> ARPCIPKSFGYSSVVCVCNATYCDSFDPPTFPALGTFSRYESTRSGRRMELSMGPIQANHTGTGLLLTLQPEQKFQKVKGFGGAMTDAAALNILALSPPAQNLLLKSYFSEEGIGYNIIRVPMASCDFSIRTYTYADTPDDFQLHNFSLPEEDTKLKIPLIHRALQLAQRPVSLLASPWTSPTWLKTNGAVNGKGSLKGQPGDIYHQTWARYFVKFLDAYAEHKLQFWAVTAENEPSAGLLSGYPFQCLGFTPEHQRDFIARDLGPTLANSTHHNVRLLMLDDQRLLLPHWAKVVLTDPEAAKYVHGIAVHWYLDFLAPAKATLGETHRLFPNTMLFASEACVGSKFWEQSVRLGSWDRGMQYSHSIITNLLYHVVGWTDWNLALNPEGGPNWVRNFVDSPIIVDITKDTFYKQPMFYHLGHFSKFIPEGSQRVGLVASQKNDLDAVALMHPDGSAVVVVLNRSSKDVPLTIKDPAVGFLETISPGYSIHTYLWRRQ

Gaucher disease (GD) is the most common lysosomal storage disorder which is caused by inherited deficiencies in β‐glucocerebrosidase (glucosylceramidase, GCase, GBA, EC 3.2.1.45). GBA is primarily responsible for catalyzing the degradation of GlcCer by hydrolytic cleavage of the β‐glucose moiety from the aglycone to yield free ceramide and glucose. This is achieved with retention of β‐anomeric stereochemistry of the released glucose unit through a Koshland double displacement mechanism using Glu340 as the catalytic nucleophile and Glu235 as the catalytic acid‐base. Here, we report the design, synthesis, and structural analysis of a range of cyclophellitol epoxide and aziridine inactivators and activity‐based probes (ABPs) for human β‐glucocerebrosidase (GBA).

Consequently, the O6−Cy5 tagged N‐octyl bifunctional aziridine ABP 6 was synthesised and its GBA activity and selectivity were compared to the parent Cy5 tagged cyclophellitol aziridine ABP 8 and cyclophellitol epoxide ABP 9. To investigate the accommodation of the two functionalities of ABP 6 by GBA, a co‐crystal structure in complex with bi‐functional ABP 6 was obtained at 1.80 Å resolution, demonstrating covalent binding of the cyclophellitol aziridine to the catalytic nucleophile of GBA. Specifically, the reacted cyclophellitol adopts the expected 4C1 chair conformation, with a covalent bond length of 1.47 Å to Glu340. Furthermore, unambiguous electron density for the ring opened N‐alkyl aziridine warhead was observed, allowing the first 5 carbons of the N‐octyl chain to be modelled. This was sufficient to establish binding of the N‐alkyl chain to the narrow active site channel formed by Gln284, Tyr313, Lys346 and Trp348, which is consistent with the complex of N‐acyl aziridine 3. In fact, the N‐alkyl chain of ABP 6 extends through this pocket towards the surface of the protein, which may provide some indication into the binding of the fatty acid portion of the natural GlcCer substrate which is thought to project out from the protein and interact with the lipid bilayer. Unfortunately, whilst sufficient electron density for the O6‐triazole linker and subsequent amide group was observed, the Cy5 tag could not be modelled. Nevertheless, the O6‐triazole linker was found to bind in the hydrophobic cavity formed by Trp348, Phe246 and Tyr313, which we reported previously to accommodate the triazole linker of ABP 9. Additionally, this binding cavity extends towards the broader hydrophobic allosteric site at the dimer interface where we reported the BODIPY tag of ABP 5 to bind. Therefore, despite demonstrating that the O6‐ and aziridine nitrogen substituents of ABP 6 are structurally exclusive and are accommodated by GBA in two unique active site clefts, ABP 6 exhibits no further improvements in potency or selectivity for GBA over the O6 mono‐functionalized ABPs.>MTKQYKNYVNGEWKLSENEIKIYEPASGAELGSVPAMSTEEVDYVYASAKKAQPAWRALSYIERAAYLHKVADILMRDKEKIGAILSKEVAKGYKSAVSEVVRTAEIINYAAEEGLRMEGEVLEGGSFEAASKKKIAVVRREPVGLVLAISPFNYPVNLAGSKIAPALIAGNVIAFKPPTQGSISGLLLAEAFAEAGLPAGVFNTITGRGSEIGDYIVEHQAVNFINFSGSTGIGERIGKMAGMRPIMLELGGKDSAIVLEDADLELTAK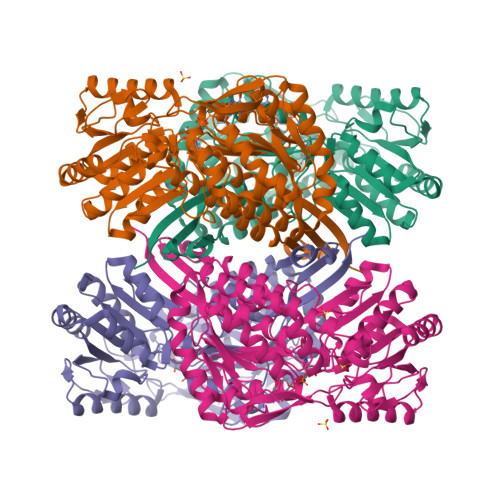NIIAGAFGYSGQRCTAVKRVLVMESVADELVEKIREKVLALTIGNPEDDADITPLIDTKSADYVEGLINDANDKGATALTEIKREGNLICPILFDKVTTDMRLAWEEPFGPVLPIIRVTSVEEAIEISNKSEYGLQASIFTNDFPRAFGIAEQLEVGTVHINNKTQRGTDNFPFLGAKKSGAGIQGVKYSIEAMTTVKSVVFDIK[4x]>TSSANEDMPVERILEAELAVEPKTETYVEANMGLNPSSPNDPVTNICQAADKQLFTLVEWAKRIPHFSELPLDDQVILLRAGWNELLIASFSHRSIAVKDGILLATGLHVHRNSAHSAGVGAIFDRVLTELVSKMRDMQMDKTELGCLRAIVLFNPDSKGLSNPAEVEALREKVYASLEAYCKHKYPEQPGRFAKLLLRLPAL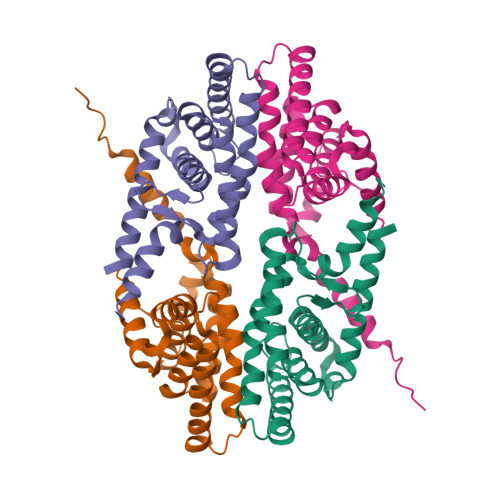RSIGLKCLEHLFFFKLIGDTPIDTFLMEMLEAPHQMT[2x]>MHHHHHHHHHHSSGLVPRGSHRILNLVKYDLYSIFKSPLTYLAILVVSSLIATQSILMANSMDNPKHIIVYGSVFAAAKWLLLIIGLMFVVKTITRDFSQGTIQLYMSKVKTRVGYIISKTISIILISILFALIHYVILIVVQASSNGKNLAFSKYVDNLWFFLIFLLFFGLFLFLITLASQKTAMIFSLGVFLVLIVPFIKPFITFIPRYGEKVLDAFDYIPFAYLTDKMISSNFDFSNWQWVISLGSIVIFFILNILYVAKKDI[2x];>MKLEHITKKYGSNVVLNDIDFDFGDSRIVGLIGKNGVGKTTVMKVMNGNIIKFDGKVDIDNADNIGFLIEHPKLYDNKSGLYNLKLFAQVLGKGFDKAYTDKIIDAFGMRPYIKKKVKKYSMGMKQKLAIAVSLMNKPKFLILDEPTNGMDPDGSIDVLTTIKSLVNELDMRILISSHKLEDIELICDRAVFLRDGHFVQDVNMEEGVASDTTIVTVDHKDFDRTEKYLAEHFQLQNVDKADGHLMINAQKNYQVILKALSELDIYPKYIET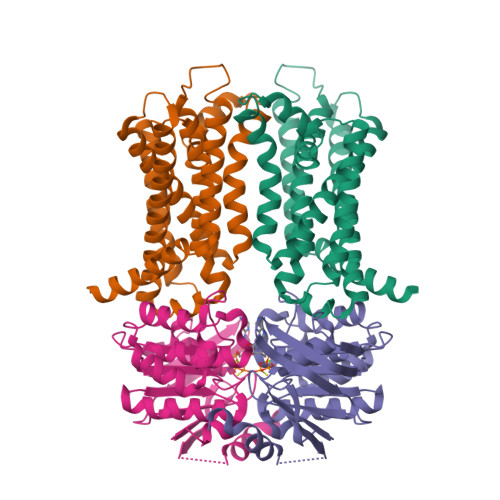RKSSLRDTYFNINQRGDK[2x]>MTEQKALVKRITNETKIQIAISLKGGPLAIEHSIFPEKEAEAVAEQATQSQVINVHTGIGFLDHMIHALAKHSGWSLIVECIGDLHIDDHHTTEDCGIALGQAFKEALGAVRGVKRFGSGFAPLDEALSRAVVDLSNRPYAVVELGLQREKVGDLSCEMIPHFLESFAEASRITLHVDCLRGKNDHHRSESAFKALAVAIREATSPN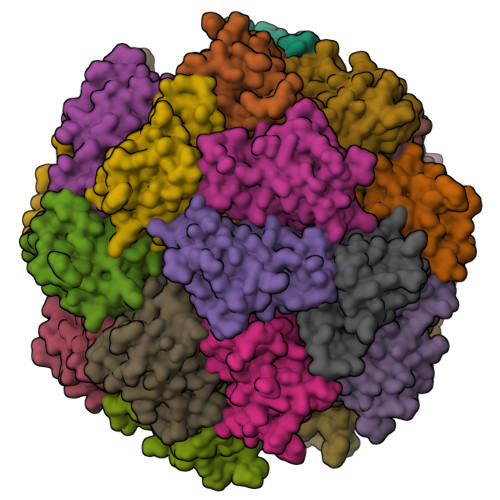GTNDVPSTKGVLM[24x]>MARRILVVEAEAPIREMVCFVLEQN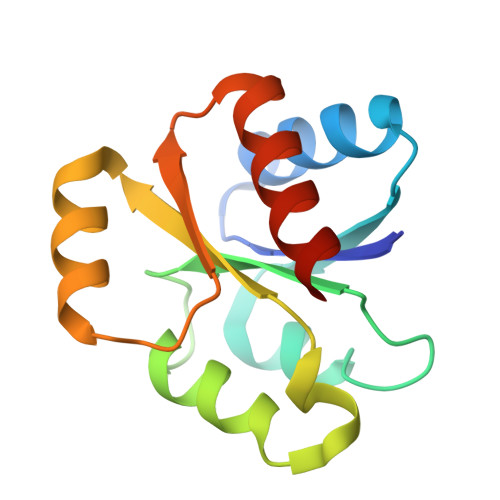GFQPVEAEDYDSAVNQLNEPWPDLILLEWMLPGGSGIQFIKHLKRESMTRDIPVVMLTARGEEEDRVRGLETGADDYITKPFSPKELVARIKAVMRRISPMA[2x]> HHHHHHMNTINIAKNDFSDIELAAIPFNTLADHYGERLAREQLALEHESYEMGEARFRKMFERQLKAGEVADNAAAKPLITTLLPKMIARINDWFEEVKAKRGKRPTAFQFLQEIKPEAVAYITIKTTLACLTSADNTTVQAVASAIGRAIEDEARFGRIRDLEAKHFKKNVEEQLNKRVGHVYKKAFMQVVEADMLSKGLLGGEAWSSWHKEDSIHVGVRCIEMLIESTGMVSLHRQNAGVVGQDSETIELAPEYAEAIATRAGALAGISLMFQPCVVPPKPWTGITGGGYWANGRRPLALVRTHSKKALMRYEDVYMPEVYKAINIAQNTAWKINKKVLAVANVITKWKHCPVEDIPAIEREELPMKPEDIDMNPEALTAWKRAAAAVYRKDKARKSRRISLEFMLEQANKFANHKAIWFPYNMDWRGRVYAVSMFNPQGNDMTKGLLTLAKGKPIGKEGYYWLKIHGANCAGVDKVPFPERIKFIEENHENIMACAKSPLENTWWAEQDSPFCFLAFCFEYAGVQHHGLSYNCSLPLAFDGSCSGIQHFSAMLRDEVGGRAVNLLPSETVQDIYGIVAKKVNEILQADAINGTDNEVVTVTDENTGEISEKVKLGTKALAGQWLAYGVTRSVTKRSVMTLAYGSKEFGFRQQVLEDTIQPAIDSGKGLMFTQPNQAAGYMAKLIWESVSVTVVAAVEAMNWLKSAAKLLAAEVKDKKTGEILRKRCAVHWVTPDGFPVWQEYKKPIQTRLNLMFLGQFRLQPTINTNKDSEIDAHKQESGIAPNFVHSQDGSHLRKTVVWAHEKYGIESFALIHDSFGTIPADAANLFKAVRETMVDTYESCD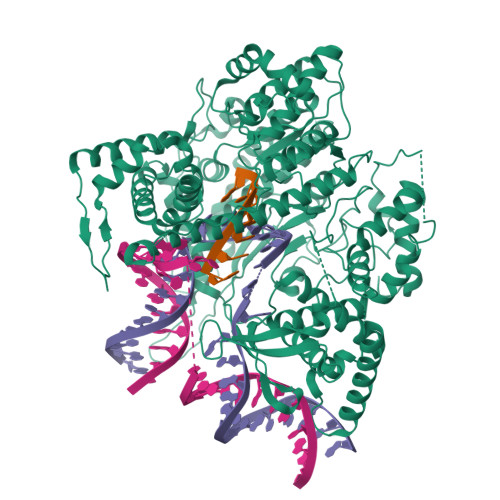VLADFYDQFADQLHESQLDKMPALPAKGNLNLRDILESDFAFA> GIDPNRIVALEWLPVELLLALGIVPYGVADTINYRLWVSEPPLPDSVIDVGLRTEPNLELLTEMKPSFMVWSAGYGPSPEMLARIAPGRGFNFSDGKQPLAMARKSLTEMADLLNLQSAAETHLAQYEDFIRSMKPRFVKRGARPLLLTTLIDPRHMLVFGPNSLFQEILDEYGIP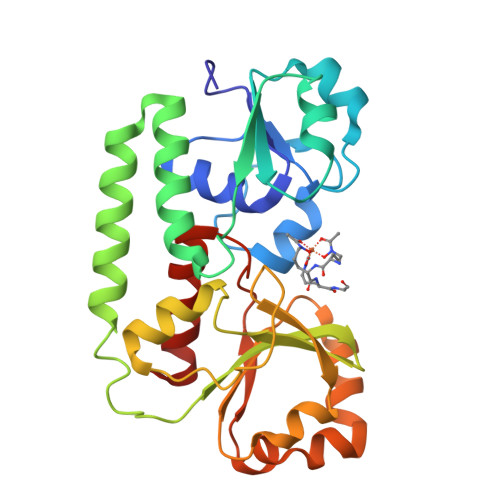NAWQGETNFWGSTAVSIDRLAAYKDVDVLCFDHDNSKDMDALMATPLWQAMPFVRAGRFQRVPAVWFYGATLSAMHFVRVLDNAIGGKA>AQYEDGKQYTTLEKPVAGAPQVLEFFSFFCPHAYQFEEVLHISDNVKKKLPEGVKMTKYHVNFMGGDLGKDLTQAWAVAMALGVEDKVTVPLFEGVQKTQTIRSASDIRDVFINAGIKGEEYDAAWNSFVVKSLVAQQEKAAADVQLRGVPAMFVNGKYQLNPQGMDTSNMDVFVQQYADTVKYLSEKK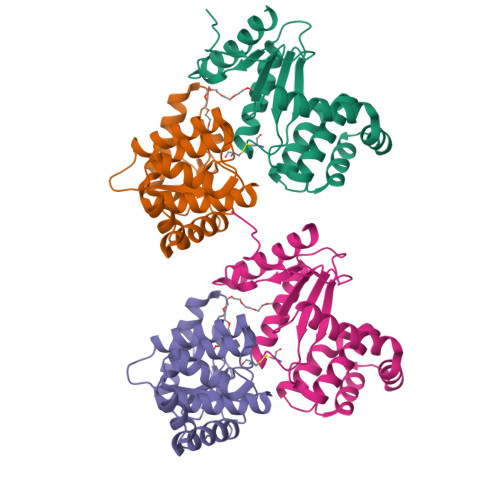[4x]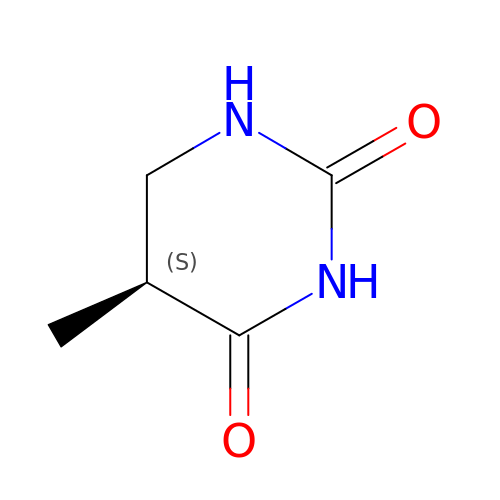(5S)-5-methyl-1,3-diazinane-2,4-dione | C5 H8 N2 O2 | NBAKTGXDIBVZOO-VKHMYHEASA-N> SESPWIAEDTSQIQTKLLEFAKSPEVFDWMVKIRRKIHENPELGYEELETSKLIRSELELIGIKYRYPVAITGVIGYIGTGEPPFVALRADMDALPIQEGVEWEHKSKIAGKMHACGHDGHVTMLLGAAKILHEHRHHLQGTVVLIFQPAEEGLSGAKKM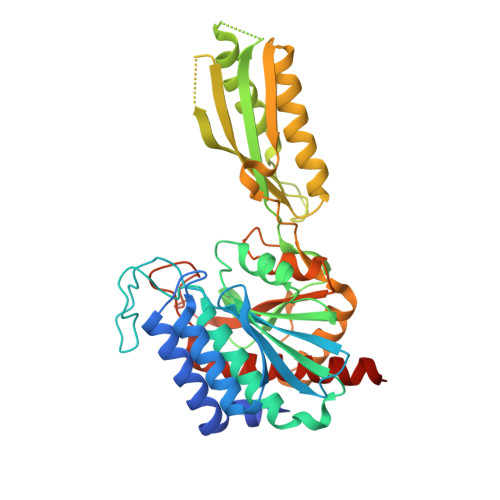REEGALKNVEAIFGIHLSARIPFGKAASRAGSFLAGAGVFEAVITGKGGHAAIPQHTIDPVVAASSIVLSLQQLVSRETDPLDSKVVTVSKVNGGNAFNVIPDSITIGGTLRAFTGFTQLQQRVKEVITKQAAVHRCNASVNLTPNGREPMPPTVNNKDLYKQFKKVVRDLLGQEAFVEAAPVMGSEDFSYFAETIPGHFSLLGMQDETNGYASSHSPLYRINEDVLPYGAAIHASMAVQYLKEKASKGSVSGFHEEL> MSQPDATPFDYILSGGTVIDGTNAPGRLADVGVRGDRIAAVGDLSASSARRRIDVAGKVVSPGFIDSHTHDDNYLLKHRDMTPKISQGVTTVVTGNCGISLAPLAHANPPAPLDLLDEGGSFRFARFSDYLEALRAAPPAVNAACMVGHSTLRAAVMPDLRREATADEIQAMQALADDALASGAIGI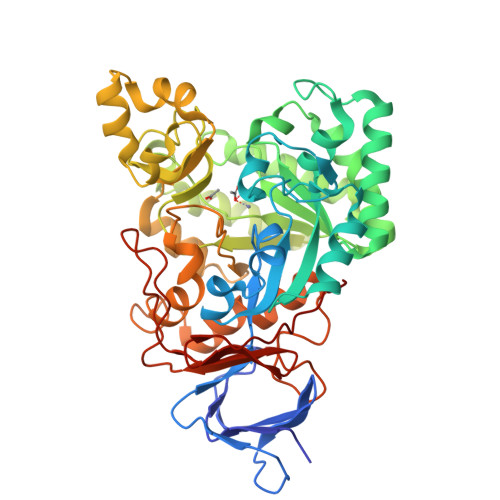STGAFYPPAAHASTEEIIEVCRPLITHGGVYATHMRDEGEHIVQALEETFRIGRELDVPVVISHHKVMGKLNFGRSKETLALIEAAMASQDVSLDAYPYVAGSTMLKQDRVLLAGRTLITWCKPYPELSGRDLEEIAAERGKSKYDVVPELQPAGAIYFMMDEPDVQRILAFGPTMIGSDGLPHDERPHPRLWGTFPRVLGHYSRDLGLFPLETAVWKMTGLTAAKFGLAERGQVQPGYYADLVVFDPATVADSATFEHPTERAAGIHSVYVNGAAVWEDQSFTGQHAGRVLNRAGA> MDSDEHLYKLKTFLENLRRHLDRLDKHIKQLRDILSENPEDERVKDAIDLSERSVRIVKTVIKIFEDSVRKKEKRPIDKR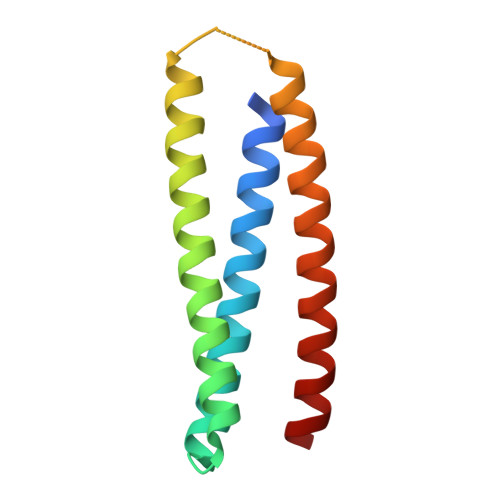DDKELDKLLDTLEKILQTATKIIDDANKLLEYLRR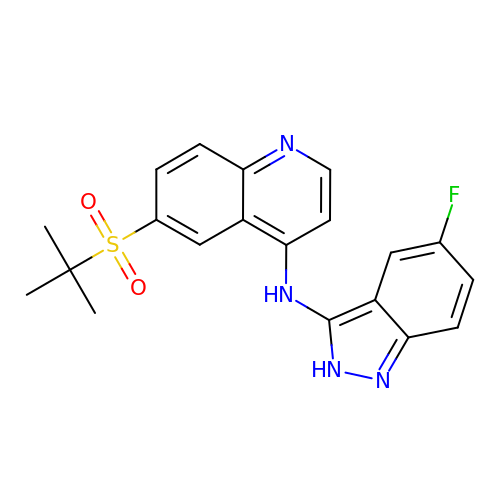6-(tert-butylsulfonyl)-N-(5-fluoro-2H-indazol-3-yl)quinolin-4-amine | C20 H19 F N4 O2 S | XLOGLWKOHPIJLV-UHFFFAOYSA-N{4-[3-(4-{[(2R)-2-hydroxy-3,3-dimethylbutyl]oxy}-3-methylphenyl)pentan-3-yl]-2-methylphenoxy}acetic 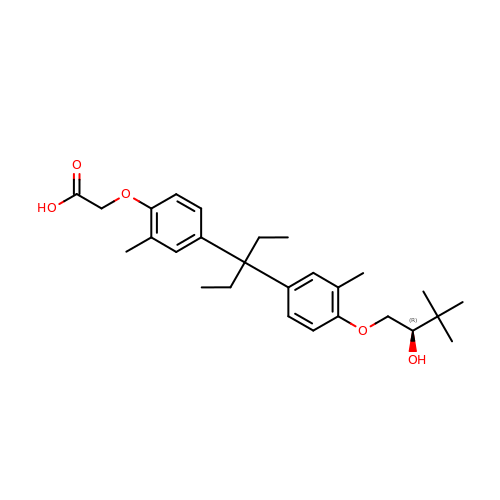acid | C27 H38 O5 | PMGXXWMCGADHQY-DEOSSOPVSA-N> TELKKVVALYDYMPMNANDLQLRKGEEYFILEESNLPWWRARDKNGQEGYIPSNYITEAEDSIEMYEWYSKHMTRSQAEQLL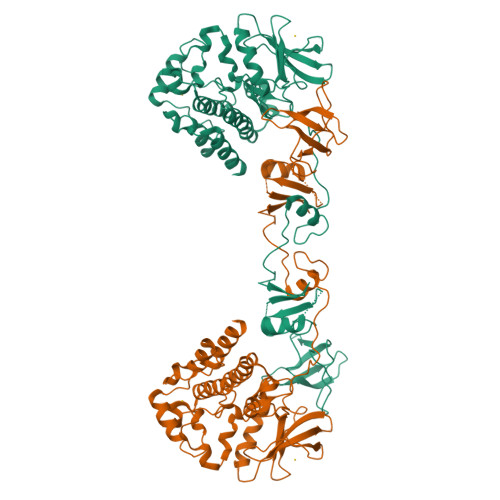KQEGKEGGFIVRDSSKAGKYTVSVFAKSTGEPQGVIRHYVVCSTPQSQYYLAEKHLFSTIPELINYHQHNSAGLISRLKYPVSKQNKNAPSTAGLGYGSWEIDPKDLTFLKELGTGQFGVVKYGKWRGQYDVAIKMIREGSMSEDEFIEEAKVMMNLSHEKLVQLYGVCTKQRPIFIITEYMANGCLLNYLREMRHRFQTQQLLEMCKDVCEAMEYLESKQFLHRDLAARNCLVNDQGVVKVSDFGLSRYVLDDEYTSSVGSKFPVRWSPPEVLMYSKFSSKSDIWAFGVLMWEIYSLGKMPYERFTNSETAEHIAQGLRLYRPHLASERVYTIMYSCWHEKADERPSFKILLSNILDVMDEES> GPDSMAPPVRYCIPGERLCNLEEGSPGSGTYTRHGYIFSSLAGCLMKSSENGALPVVSVVRETESQLLPDVGAIVTCKVSSINSRFAKVHILYVGSMPLKNSFRGTIRKEDVRATEKDKVEIYKSFRPGDIVLAKVISLGDAQSNYLLTTAENELGVVVAHSESGIQMVP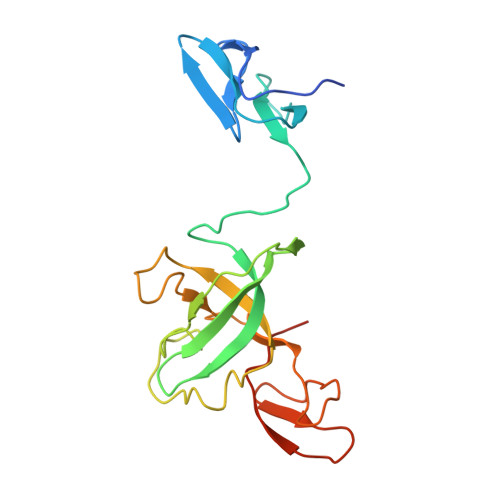ISWCEMQCPKTHTKEFRKVARVQPEFLQT> GELRVGLEESELWLRFKELTNEMIVTKNGRRMFPVLKVNVSGLDPNAMYSFLLDFVAADNHRWKYVNGEWVPGGKPEPQAPSCVYIHPDS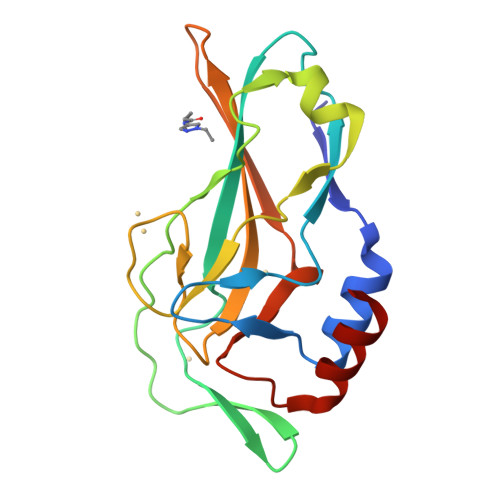PNFGAHWMKAPVSFSKVKLTNKLNGGGQIMLNSLHKYEPRIHIVRVGGPQRMITSHCFPETQFIAVTAYQNEEITALKIKYN>[2x]MAQLKADLSNLEECLPSTLSQEQRAVAKTQFYKELAEKVHKFYKGKIQIMPKCTLAGFNWFNAYYTPGVSRISTNIRDNNDSSLFYSLRGNFVGVVSDSTRVLGDGDVTPPGGLGVMEGKALLMKYLGGIDAVPICIDSKNKEGKNDPDAVIEFVQRIQHTFGAINLEDISQPNCYKILDVLRESCDIP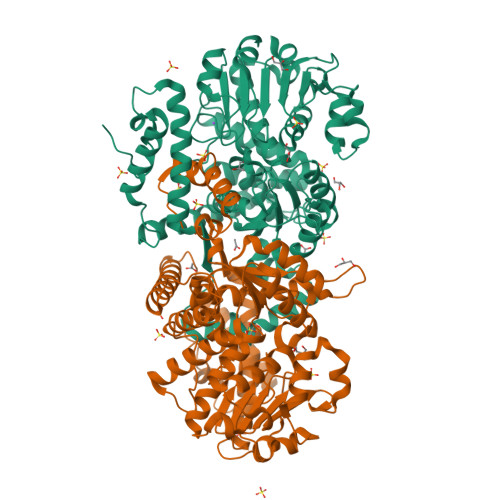VWHDDQQGTASVTLAGLLNALKLVKKDIHECRMVFIGAGSSNTTCLRLIVTAGADPKKIVMFDSKGSLHNGREDIKKDTRFYRKWEICETTNPSKFGSIAEACVGADVLISLSTPGPGVVKAEWIKSMGEKPIVFCCANPVPEIYPYEAKEAGAYIVATGRGDFPNQVNNSVGFPGILKGALIVRARKITDNMAIAASRALAEFAEKRGINPDNIIGTMDEPGIFPKEAADVAMQAIKDGVARVTDLTWQQVYDIAEHDIKEARESAQLLQDSKHIVDFPQETLNECLAYAINKVTGK>[5x]MSFNSPFFDFFDNINNEVDAFNRLLGEGGLRGYAPRRQLANTPAKDSTGKEVARPNNYAGALYDPRDETLDDWFDNDLSLFPSGFGFPRSVAVPVDILDHDNNYELKVVVPGVKSKKD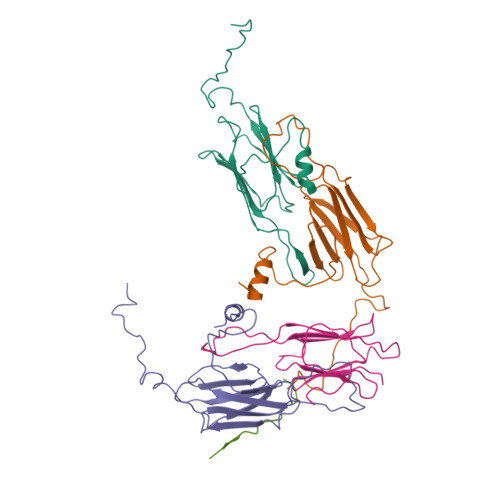IDIEYHQNKNQILVSGEIPSTLNEESKDKVKVKESSSGKFKRVITLPDYPGVDADNIKADYANGVLTLTVPKLKPQKDGKNHVKKIEVSSQESWGN>MVLYFIGLGL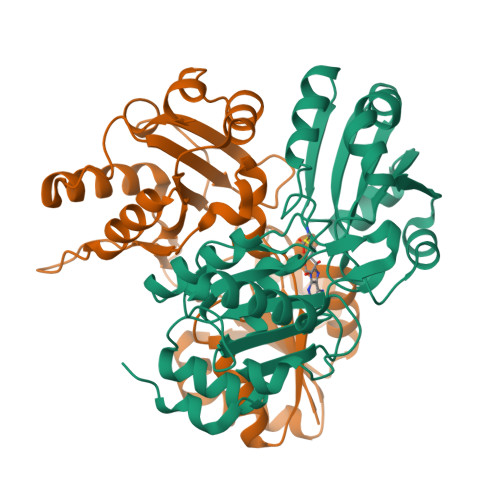YDERDITVKGLEIAKKCDYVFAEFYTSLMAGTTLGRIQKLIGKEIRVLSREDVELNFENIVLPLAKENDVAFLTPGDPLVATTHAELRIRAKRAGVESYVIHAPSIYSAVGITGLHIYKFGKSATVAYPEGNWFPTSYYDVIKENAERGLHTLLFLDIKAEKRMYMTANEAMELLLKVEDMKKGGVFTDDTLVVVLARAGSLNPTIRAGYVKDLIREDFGDPPHILIVPGKLHIVEAEYLVEIAGAPRMILRVNV[2x]>[2x]MPKVILKGPLISQFNFREIYVNDRELLRVLVKIDSKKHLILNESNQ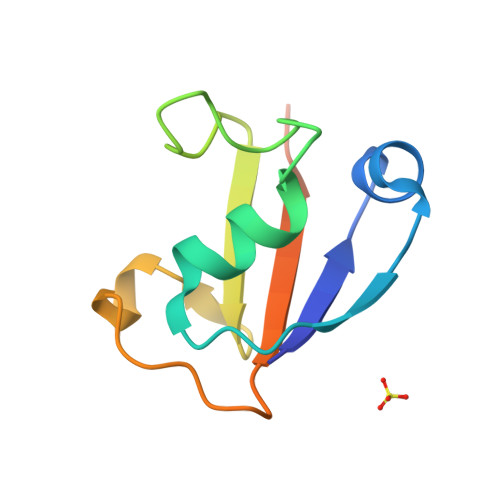LKSGILILINGKDWRLYRNQLLNDNDIIEIIPINHGGLEHHHHHH> MTSKVYDPEQRKRMITGPQWWARCKQMNVLDSFINYYDSEKHAENAVIFLHGNATSSYLWRHVVPHIEPVARCIIPDLIGMGKSGKSGNGSYRLLDHYKYLTAWFELLNLPKKIIFVGHDWGAALAFHYAYEHQDRIKAIVHMESVVDVIESWDEWPDIEEDIALIKSEEGEKMVLENNFFVETVLPSKIMRKLEPEEFAAYLEPFKEKGEVRRPTLSWPREIPLVKGGKPDVVQIVRNYNAYLRASDDLPKLFIESDPGFFSNAIVEGAKKFPNTEFVKVKGLHFLQEDAPDEMGKYIKSFVE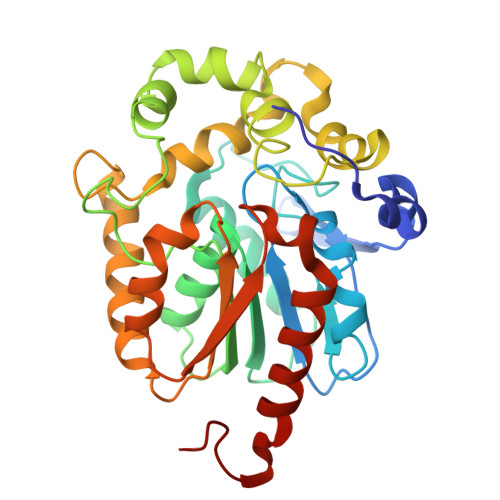RVLKNEQSGLEVLFQ(2R,3R,4R,5R,6S)-2-(aminomethyl)-6-methylpiperidine-3,4,5-triol 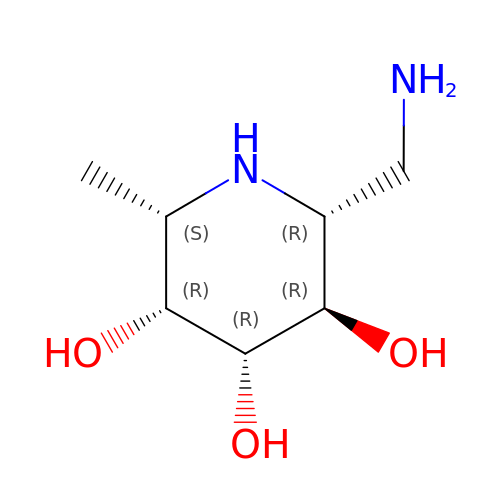| C7 H16 N2 O3 | AKIVXVRDQKFDJC-CQOGJGKDSA-N> MSTFIFPGDSFPVDPTTPV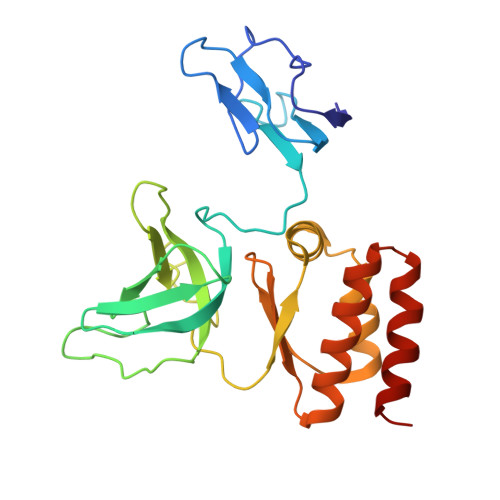KLGPGIYCDPNTQEIRPVNTGVLHVSAKGKSGVQTAYIDYSSKRYIPSVNDFVIGVIIGTFSDSYKVSLQNFSSSVSLSYMAFPNASKKNRPTLQVGDLVYARVCTAEKELEAEIECFDSTTGRDAGFGILEDGMIIDVNLNFARQLLFNNDFPLLKVLAAHTKFEVAIGLNGKIWVKCEELSNTLACYRTIMECCQKNDTAAFKDIAKRQFKEILTVKEE>PNFSGNWKIIRSENFEELLKVLGVNVMLRKIAVAAASKPAVEIKQEGDTFYIKTSTTVRTTEINFKV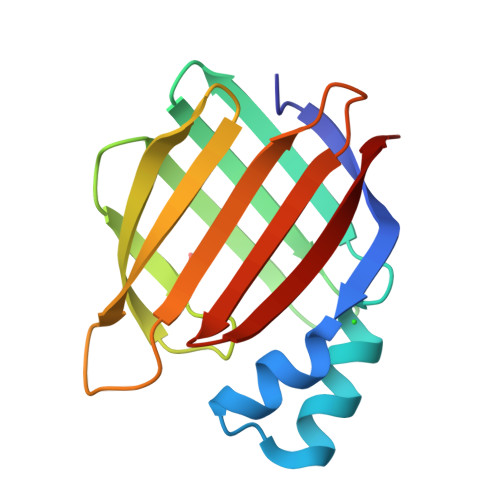GEEFEEQTVDGRPCKSLVKWESENKMVCEQKLLKGEGPKTSWTRELTNDGELILTMTADDVVCTRVYVRE[2x]> GAEFMALPRLTGALRSFSNVTKQDNYNEEVADLKIKRSKLHEQVLDLGLTWKKIIKFLNEKLEKSKMQSINEDLKDILHAAKQIVGTDNGREAIESGAAFLFMTFHLKDSVGHKETKAIKQMFGPFPSSSATAACNATNRIISHFSQDDLTALVQMTEKEHGDRVFFGKNLAFSFDMHDLDHFDELPINGETQKTISLDYKKFLNEHLQEA;> GAMAMPALPLDQLQITHKDPKTGKLRTSPALHPEQKADRYFVLYKPPPKDNIPALVEEYLERATFVANDLDWLLALPHDKFWCQVIFDETLQKCLDSYLRYVPRKFDEGVASAPEVVDMQKRLHRSVFLTFLRMSTHKESKDHFISPSAFGEILYNNFLFDIPKILDLCVLFGKGNSPLLQKMIGNIFTQQPSYYSDLDETLPTILQVFSNILQHCGLQGDGANTTPQKLEERGRLTPSDMPLLELKDIVLYLCDTCTTLWAFLDIFPLACQTFQKHDFCYRLASFYEAAIPEMESAIKKRRLEDSKLLGDLWQRLSHSRKKLMEIFHIILNQICLLPILESSCDNIQGFIEEFLQIFSSL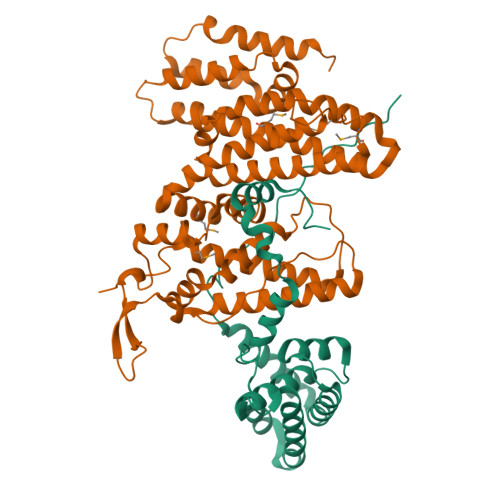LQEKRFLRDYDALFPVAEDISLLQQASSVLDETRTAYILQAVESAWEGVDRRKATDAKDPSVIEEPNGEPNGVTVTA>SGAVQLRFDNTYDNASGSMNTVACSTGANGLSQRFPTFGSVPTFPHIGASSDIGGFNSPACGNCYTISFTFQGVTRSINLVAIDHAGNGFNVAQAAMDELTNGNAVALGTIDVQSQQVARSVCGL[2x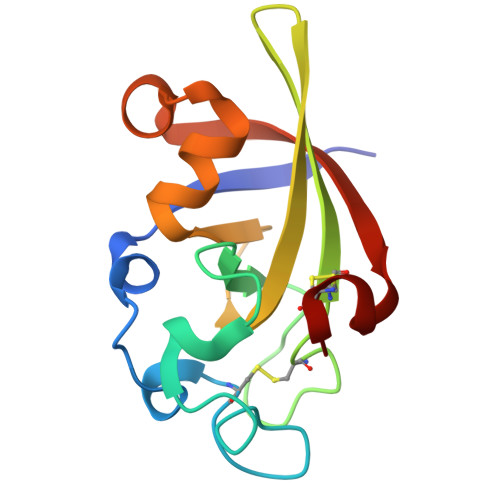]>[4x]LVASGENKIKQGLLPSLEDLLFYTIAEGQEKIPVHKFITALKSTGLRTSDPRLKECMDMLRLTLQTTSDGVMLDKDL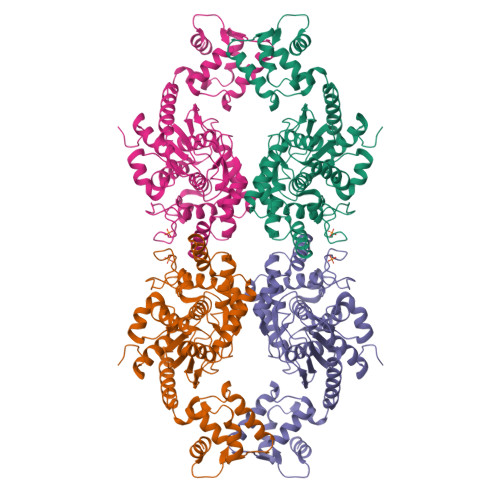FKKCVQSNIVLLTQAFRRKFVIPDFMSFTSHIDELYESAKKQSGGKVADYIPQLAKFSPDLWGVSVCTVDGQRHSTGDTKVPFCLQSCVKPLKYAIAVNDLGTEYVHRYVGKEPSGLRFNKLFLNEDDKPHNPMVNAGAIVVTSLIKQGVNNAEKFDYVMQFLNKMAGNEYVGFSNATFQSERESGDRNFAIGYYLKEKKCFPEGTDMVGILDFYFQLCSIEVTCESASVMAATLANGGFCPITGERVLSPEAVRNTLSLMHSCGMYDFSGQFAFHVGLPAKSGVAGGILLVVPNVMGMMCWSPPLDKMGNSVKGIHFCHDLVSLCNFHNYDNLRHFAKKLDPRREGGDQRHSFGPLDYESLQQELALKETVWKKVSPESNEDISTTVVYRMESLGEKS>MAKNTITKTLKLRIVRPYNSAEVEKIVADEKNNREKIALEKNKDKVKEACSKHLKVAAYCTTQVERNACLFCKARKLDDKFYQKLRGQFPDAVFWQEISEIFRQLQKQAAEIYNQSLIELYYEIFIKGKGIANASSVEHYLSDVCYTRAAELFKNAAIASGLRSKIKSNFRLKELKNMKSGLPTTKSDNFPIPLVKQKGGQYTGFEISNHNSDFIIKIPFGRWQVKKEIDKYRPWEKFDFEQVQKSPKPISLLLSTQRRKRNKGWSKDEGTEAEIKKVMNGDYQTSYIEVKRGSKICEKSAWMLNLSIDVPKIDKGVDPSIIGGIDVGVKSPLVCAINNAFSRYSISDNDLFHFNKKMFARRRILLKKNRHKRAGHGAKNKLKPITILTEKSERFRKKLIERWACEIADFFIKNKVGTVQMENLESMKRKEDSYFNIRLRGFWPYAEMQNKIEFKLKQYGIEIRKVAPNNTSKTCSKCGHLNNYFNFEYRKKNKFPHFKCEKCNFKENADYNAALNISNPKLKSTKEEP[2x]

Cas12f, also known as Cas14, is an exceptionally small type V-F CRISPR–Cas nuclease that is roughly half the size of comparable nucleases of this type. Cas12f associates with a crRNA and a tracrRNA, which can be fused into a single guide RNA (sgRNA), to target substrate DNA. An asymmetric Cas12f dimer is bound to one sgRNA for recognition and cleavage of dsDNA substrate with a T-rich PAM sequence. Despite its small size, Cas12f contains all the conventional domains of Cas12 proteins, compared with other known Cas12 nuclease structures.

We assembled a Cas12f–sgRNA–target DNA ternary complex by incubating an inactive Un1Cas12f1D510A (529 amino acids or a.a., 61.5 kDa)(10), a sgRNA (222 nucleotides), and a target dsDNA with a TTTA PAM sequence (60 bp). Using cryo-EM, we determined the structure of this complex at 3.1 Å resolution. The most astonishing feature of the structure is the presence of two copies of Cas12f in the complex (named Cas12f.1 and Cas12f.2), in contrast to all previous determined structures of other class 2 effectors. The PAM sequence is recognized at the interface of REC1C and the WED domain. The PAM proximal end of the heteroduplex is primarily recognized by Cas12f.1, whereas the PAM distal end is bound to Cas12f.2. Interestingly, the lid motif in Cas12f.1 is in an open conformation, in correspondence to the crRNA–target DNA heteroduplex formation. However, the lid motif in Cas12f.2 is in a closed conformation, although this active site is closer to the 5′ end of the target strand. Two purine bases from the Stem 2 of tracrRNA, G(24) and A(62), insert into the inactive RuvC catalytic pocket, likely further inhibiting substrate access. Interestingly, we observed an extended density assigned as the substrate DNA trapped in the RuvC active site of Cas12f.1, likely from excess DNA oligos used in complex assembly. The rotation of C(4) and the close proximity to the triplet of acidic residues indicate the phosphate group connecting C(3) and C(4) is the scissile phosphate targeted for cleavage.> M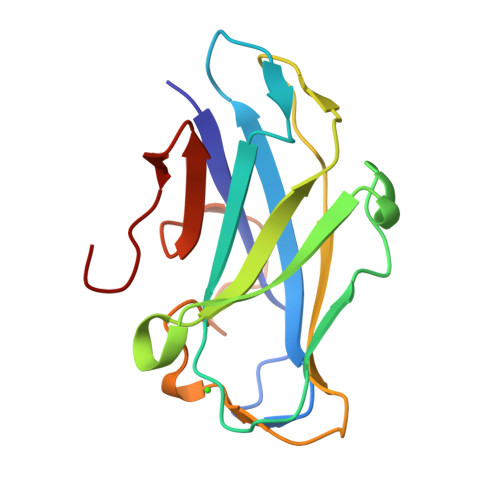DVKVQYLCENTQTSTQEIKGKFNIVNTGNRDYSLKDIVLRYYFTKEHNSQLQFICYYTPIGSGNLIPSFGGSGDEHYLQLEFKDVKLPAGGQTGEIQFVIRYADWSFHDQSNDYSFDPTIKAFQDYGKVTLYKNGELVWGTPPGG> GPGSEFGEVVDCHLSDMLQQLHSVNASKPSERGLVRQEEAEDPAC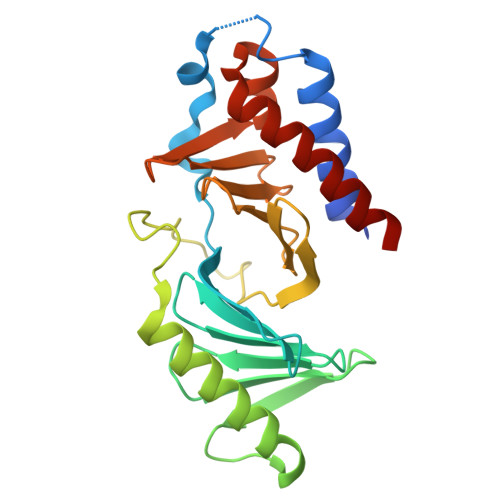IPIFWVSKWVDYSDKYGLGYQLCDNSVGVLFNDSTRLILYNDGDSLQYIERDGTESYLTVSSHPNSLMKKITLLKYFRNYMSEHLLKAGANITPREGDELARLPYLRTWFRTRSAIILHLSNGSVQINFFQDHTKLILCPLMAAVTYIDEKRDFRTYRLSLLEEYGCCKELASRLRYARTMVDKLLSSR>[2x]ETGGSWAQVKLLESGGKVTHEGQSVTLTCKASGFNFKDYAMSWHWNPSGSNRQFVASISPKTGSKREYKPSIQGRALITRNNEANTVSLTLRQLRKEDSGIYYCAKPSGLRQWGPKWEPLAEQWENFGPGTELTVLPLEKTLLTESGGGTYQAGKTLSLKCQTSGFQFKTSQLDWYLWTPGHAPLWLTGLNSSSTDATEGRITSSREDNKNQIFLQIEDLGLRDSGQYHCARRVGNGDDTDKLVFGLGTRVIVEPRPAAPLSPSVFLVRDQDAVACLIRNFYPKELHVSLTSSGTLISAQSLSLAPTASGTYSAIHIGRVGENDAITCSVKHLGKEIHMSHQAGSLVPR;>ETGSCAHMKQQVSFTGIQGDSARITCQVSNAVSYWIHWYRFQDGKPPQRLLCLSRESGELLFDEGFGSNKFHAFKDQFNGEKFILLIKKLEVRDSGMYYCAIWDWDGLVKVFGEGTRLIVTESAFKKKPPKPIFFLPTSEEI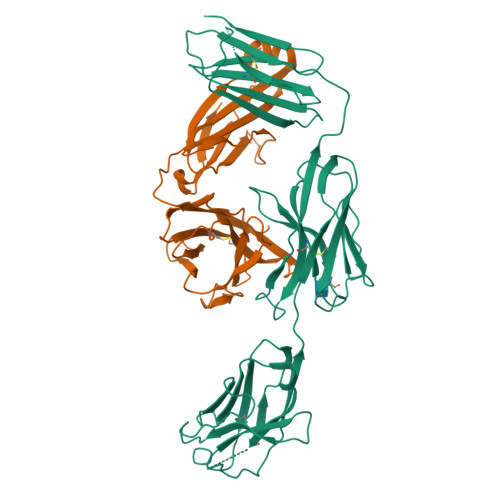KQKQSGTYICLLEDFFPNVVKTYWKEDGNSQPLDAQFGPITGGGNSYSQVSWLTVKEDVLRKNLTYFYQHEDLGMEPKAFSISSVREKGSLVPR[2x]> AAASLYE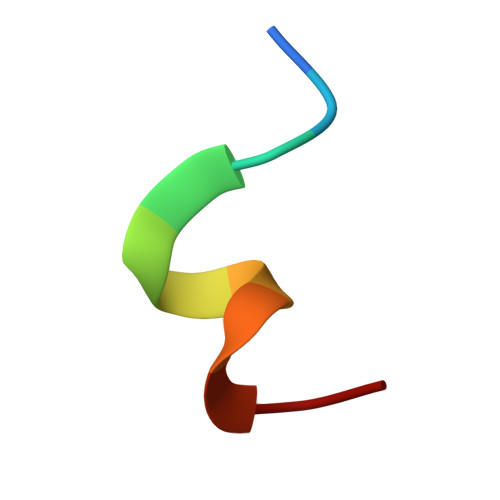KKAA> LRGSGEEEEEELVDPLTTIREHCE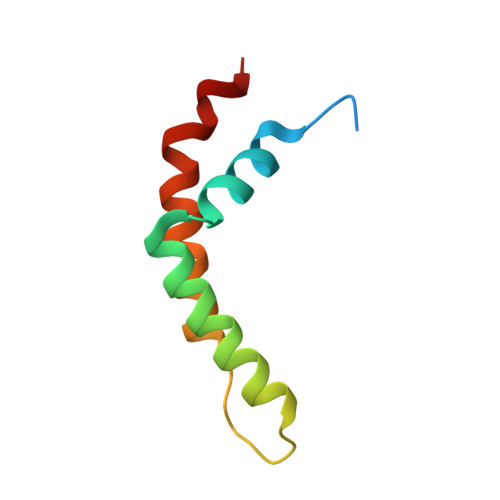QTEKCVKARERLELCDARVSSRSHTEEQCTEELFDFLHARDHCVAHKLFNKLK>S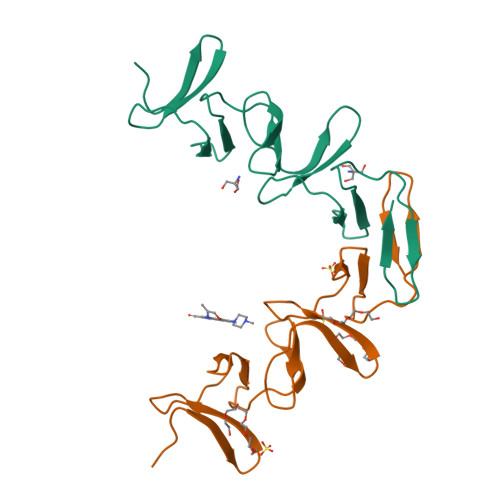YPKDKFEKINGTWYYFDSSGYMLADRWRKHTDGNWYWFDNSGEMATGWKKIADKWYYFNEEGAMKTGWVKYKDTWYYLDAKEGAMVSNAFIQSADGTGWYYLKPDGTLADRPEFTVEPDGLITVK[2x]4-phenylbenzenesulfonic acid | C12 H10 O3 S | 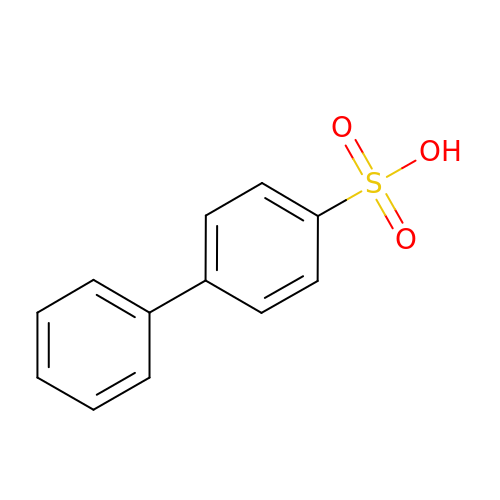XDTYUYVIGLIFCW-UHFFFAOYSA-N> HMGTGSLGGGFPGKG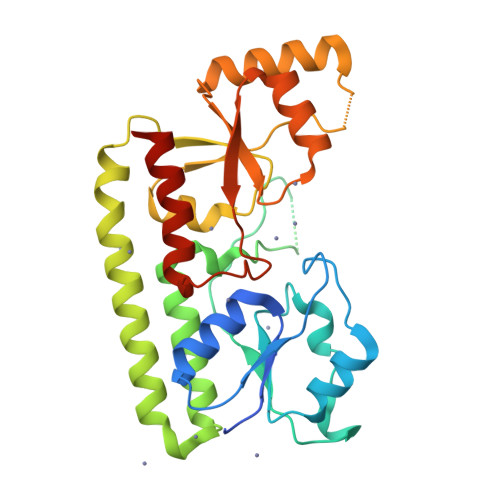MKIVTSFYPIYAMVKEVSGDLNDVRMIQSSSGIHSFEPSANDIAAIYDADVFVYHSHTLESWAGSLDPNLKKSKVKVLEASEGMTLERVPGLEDVEAGDGVDEKTLYDPHTWLDPEKAGEEAQIIADKLSEVDSEHKETYQKNAQAFIKKAQELTKKFQPKFEKATQKTFVTQLTAFSYLAKRFGLNQLGIAGISPEQEPSPRQLTEIQEFVKTYKVKTIFTESNASSKVAETLVKSTGVGLKTLNPLESDPQNDKTYLENLEENMSILAEELKGNLYFQ>[4x]MGRENVLPVHNDVYEDFVFTTPYFQPESTFKSVPKLFSDILLGGVEWVYTTSESVLAYDYKLWYLWSGVSNLDESFDMFFNQYWALSLSTSVFQLFYAVILDRYLSVLFQNTPYTNDWFRMMLHSKETALIWLYHPELSWHINGLNQFFTYFYGGILEFVYFDKSNPDMCILVHTLWIHLLILFLIFTGFVTILFSFYGNPNTEENTIDSDYLAASGTVEAEKEITSIDDYLGLVFAIAYVFGVFFYVHGWTSMLSHAVLLLSCYSIIIMFLFILGMPTLLLYDFGIFFLAYLKGAGKYISSVAEMMFDYTACLVFYIRILAQWIRVVLMVVTFISLSHYVSDFDITNSALIGSENQSDSMNELNTNFSMTYYILTVLPGKFIYWIYEILHTFFVVCSQFVAFFAIVFWLFLFLYTFFIIEKHEDFFSKKREERKKKLKELWNLKN;>[12x]MIRNFHSLVKRVPRLALTPFFGFRTSMTLADKKLSTGEASVVLAEKIKGITQQNDITEYGTVISIGDGIARVFGLTKVQAGEMVEFKSGIRGMALNLETDNVGVVVLGNDRDIKEGDVVKRTGAIVDVPIGEAMCGRVFDALGNPIDGLGPLKTTQRARVEIKAPGIIPRQSVRQPMQTGIKCVDSLVPIGRGQRELIIGDRQTGKTAIAIDTILNQKEAFNTGDVKKQLYCIYVAVGQKRSTIANLVSILKQHDCMKFTIVVCATASDAAPLQFLAPYSGCAIGEFFRDNGKHALIIYDDLSKQAVAYRQMSLLLRRPPGREAYPGDVFYLHSRLLERAAKMNDSLGGGSLTALPVIETQAGDVSAYIPTNVISITDGQIFLETELFYKGIRPAINVGLSVSRVGSAAQIKAMKKIAGNLKLTLATYRELAAFSQFGSDLDAKTQQQLNTGERLVEMLKQNQYTPMKVEEQVCIIFAGVKGFLDALVTSEVLKFEKKFLEHVRTNHSALLKRIRDSGDLSEVDTNELNTIIPLFIQEGGFKLKAQ;>MHSTLRVFTKNNCLSFTNMNRFSTAAQVAQANYSKFRADYSASVAAFQQRIKTIEKENTGSMKKPMAKAYEHPYNSEHHPLNFSAVKIAETFHDFIGPEQVSPHYESFAMSRKFLLTFWGGFFVLNFGMATVDLNWIMKSTYIPWIFWFQLMYFYVEGKNSMFMPLLQRFYRRAAANEIFTMEAFYHENIENKLRNLMRITKGQLEYWDIHTSYGEIRADSINNFLANEYLRLQSHITSRALNILKQAQAYETMNQAALLQKLIDDATSAIDNALKGDKKAEVLARSLDSAIDGLSKGYMDYQNDPLLPLILSSIEANVKKITTLSAQEQANLIGLTAEQLKSIKENDVRARKEFLESQPKLDNNLKNIESVKKILATWGK[4x];>MITILDYLFLLDLNDDLTRKAVFEQVIIFIFIYCTMNFLAWSTVVELIWPTHFFNRRHSSSQEFIRFRTYTEVLLKISAYNDFFYVLNNYYYNQKLILKN[4x];>[4x]MSMLAKIAKNVVKTQALKNTTAAQTPSFQAPGNQDKILKWISTLSNKATTGESRSYCTQLSSLVSFYNKQHVEQIPTIDFNEWKSVISTQGLVDKVKENYESLIKEQYNTDAISKQISSASSKALDDIENELSFHAAIWLNAYADYTMFLFELEEYNDPNDYLMHENFDFFRGLETELEELTETHNYIPGAKDDVNLRGYLATQFAWGKKVISFYRHPADDFKCAKATKNMLGR;>[12x]MLSKALQRGIARAFSTTAKKEAPKTVKANGQVSQVIGAVVDVQFEGELPQILNALEVQGTQHRLVLEVAQHLGDSRVRTIAMDSTEGLVRGQPVVDTGLPISVPVGPGTLGRIMNVIGEPIDQRGPIKAAKLYPIHRDAPSFTDQATSAEILVTGIKVVDLLAPYARGGKIGLFGGAGVGKTVLIQELINNVAKHHGGYSVFAGVGERTREGNDLYHEMMDSKVISVKEGESRCALIFGQMNEPPGARARVGLTGLTVAEYFRDEEGKDVLLFVDNIFRFTQACSEVSALLGRIPSAVGYQPTLATDLGALQERITTTQKGSITSVQAIYVPADDLTDPAPATTFAHLDATTVLNRGLTELGIYPAVDPLDSTSRMLDPITIGEEHYTVARGVQKLLQDYKSLQDIIAILGVDDLSEEDKLVVARARKVQKFLSQPFFMSEVFSGIPGRFVNLKQNIASFKALLEGAGDEYPESCFYMKGDLEESLAAGRADALKSK;>[4x]MIHCLRNIRTVSALQSKISYNLGGGNKRKKTSGDLDNYDVLFVGANLGGICSNHFDKDTHGKYKCFVSFDQPINQIYSVRIPYEQQRVRKSEYIHFSKKSINQFTPSEMLAVKEILPEQNAVVLSSGRRIGYNQLVLATGLKHDFSQIKGFYEALEHPEHPVYANRDPETWRSAQHKYSKYISNFKSGDGYFCIPEYPYAGEVECFNFFVSDEVWKWAQHHGALSPKHTFTIVNANEKFVHYCDSADAFIKERLEKRGIRVEYNTKLLEVHQDGQKATFINTKTGEKSVRDYNNLYSIVPSKRQEFLDKAGLTNGNGLLNVDHQTLQHKKYKNIFGLGDAADLPTTKTFWAGWYQIAVVRNNVKRNLQGQTLNAHYDGFSKVPLFTGHQTLTYVAHSYGGVGNWQHLKHNNGGILAWMRYRSWAKGMAKKFQDFYNGARLGPPYHKVLKSFPELPGSPESQQSSGISKYFPTKTENKAAH;>MSLHEKMQTDYLWVKDHSQADSWAKARTHGYNYIAHTVPNKKERYEMIWRSMGKSTDWELEKFRLGKKFPDRGNKRRWFKNLFRLIKNPMGYIFWKTYKARLAKPSLIVTSMFIGFTLGFIKLKAQSIAYSKKQYATLRAGKNIEGSGQVHFGYHDQKWGMPAIPMFQLMYYELPGNSIVVNPCRNQNYRLYFEMRKKLGILPA[4x];>[4x]MINRSTAFISKNLRQANLTQSSLAMKTQYNQMGFSSDNPYNKRWEYKWKHSYYTYPRDYEHTEVRKPQDSKDVPPIYFAYYKDFVDRWLPGMNMWWQRRHRIFDKFNVYFLPGMSLFFYQFADLALGFKIMAAFPLFLAYTRIRDKTLDPDFKETYLRDMIYQNPEITKYFNEETIHVLDYEFEYLPGYLCPEKFPEYQNKTWQFFNTDTAQAEGFFKFGDVESGATMTLKFKTMPIPGKFRYQVGEPFYFYDLRAEIKCDGVYKEVVLVDEKESLKKIRPFLFLI;>[4x]MQVIRKHLAQKGLFNPFLFNRFSTQQDITSVPGDKPPAIEDSIHGKYAGVLFSSASSNKSLNKVAEDMKYFNQLYKESEVFKSFLNNVSLKRNQQRDIISALGKTNFNPATNNLLETLIENKRLDSLPKIAEKYMDYYRILNKQESITIISAQELTAAEKQKVEQGLKKGNANVQFTVVYQVDPAILGGLQMYSGNNFLDCSLLSRVNKLKTEIAKISF;>[4x]MQQRKKIYLRQKRKIYIQLKNKEKKKNNQFIQKREKMGYKIRNKSIFWTRAGWKNNWHPKNFNAPRPSYGEFTMGIRCRNDHHSFLRYVQTYRNMSRHCKQY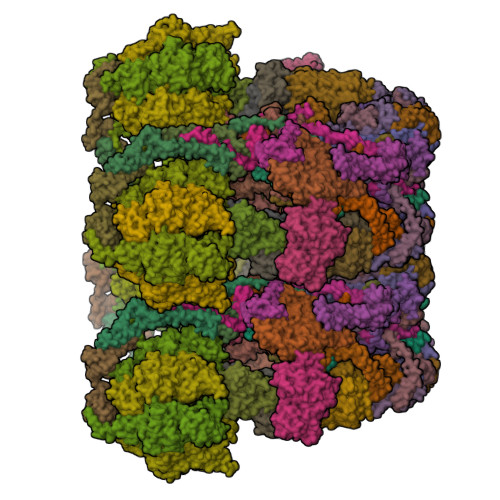FLGDKQLEETFILGLRSLFLVPYDSQCLTDQIKHGGERRFVDQLDRDFELISYNTHPYQLFTYTVRNEHLAWKNEQYEKIQKGEKTFEQELLDYLDEQVLAEKAKLRDGQNFSIERMTEIALHVFRKARAGKVRPAQDVRGPDGNVNDFLEQRRPFEHPNPTGVTH;>[40x]MLLVKAVKVLVMGGCMLPIAFGALGTGVLFAGFNVALSRNPEETESLFNNTLMGFALIETFIFMSIGLGFFVLFAA;>MNPIQKAWLKILEPVSYVINEKMAKRTGIIGKLGRFFAIGPREYGVHPINRMFIFMNRKYMAFQAVALHRYSFVKSLTHNGFHMLRVFRHFAFVLPATVLAGLGLFVYWGDDNKCYSPDRFPYLKKRAGDMALPLNSLNQRTSAHYIEINAIYGAEMMKRYHKVWENIIEERSKATDQEKKTRYAHPSYQYSPLPVVSIPNVLNPLNLQ[4x];>MSENKAPGQIYAYDIHNTHYPYVNIKQDSQTQLLASFRRSIASINPFSYRQVPSQDRAAFGLRWGNAWYAPNPYPNGIHFDRVFPTHYDPLAETNRTKANLQLIKYAPGNYSTLVVTSEKLPRPCIRTIQNYRRCQMVNGTEKCNSEAQDILAICPNWALDHMKEKVRFYTKALAINNQTYIRAMQVEEYNQGRTVADVAPKTWIHGTRQHLRPDTMWADDRYTNITQTEINEAIKRVEARKAREHEKKPVEQANVNANTGEQPVRVEKSLYP[4x];>MWYKYFSKQSWNLRVWRKANLKYNQDDFGMTQPKYIARFGDFRFRLVRTEGALRGCMFFVGFGCFSIINYLYGRYGYIINESSQKRAAQDLLDNDMAADKILFKNRVGAPTRPLRSLDDMMAFLSGSATYDQLADYASYNHAMDVNQDQQAGLDSWMSEKDKNMVKYYQRSLGKKVEGI[4x];>[4x]MPVKEGQAKLWFSTKEEADAYDDKMISNIELKSQDYEDENFSPVFNRKTQEYFLEPSEKFKSDFAELLRPLRSLSFNQVVDRYVLIPPNHTFYRNWTYEKFLGGFGLSYLILRELPLRNFYARVFVMYAFAAKVLDHLGNPFPFSGHGQIVAAADRWNHWDVRCYDNVMKALKYIRIPTVQNNIPEATRWYGRQPGHLLRADTYWIPNLVSQRFAKHQPAHWDGTQNMPIFRLADPKHKDSYMVQFR;>MDNYFTAITLLGLRDQNLPPFKDARLQRYKSIKKMIDLIETTTKLAPPMPVELFMLNPTDPEWDDDMTYPTITHATALYKSSALAGNLFLYAYNYNNFTANIRLRTMRYLFPVVSLAIFGNIYWDYRSQLVKVNLFDEYIQARAQELVKQNEYLLEHEDVKRYVWWYEDLKETLARVHRQANNHKACDFKDSEIILQDFIRRYTNPKDNLPIKFHPQGQTF[4x];>MEGFIQNKRKKEKEGEEEEESKEKRKQINQLNKQKQEEEKIYQQKKDQKRKKYLYQRKEMTIFAETWEASEYQYRNKANLKTLPVNHLGKLAELKFDFVEYKAHQLIACHLYERMTIHCMNQYGLFKDFYRPECLDAQYYFKTCVELNAAYGIQKKFFPEHFVGSPYARPVPQFQQLGL[4x];>[4x]MKQKINKLLKNKGVQDKYKYLSKLILLDQEIKGKIKRKNKKEKQKRKNKLILEEMQNTTNIVHVPVHMGHTHYFDYIDSFPKLKEGPTLEENHITNQKILREQLISGQQGLEQNLCLRNCFKLSQKRYIEFCLDRKCGGADFQRAATILGYTKN;>MSNIFLELQDGDKTVYTHTSLIEESKQEQIQAIYDKVPQWTNGGRFLGFWLSMEAVNRVQSVAKLPIYYRAGIVATSTLLGGLVSSLVFWKSGNENQVAKLANGAPVYLKKWEVPELSKLYFFLDDDNNFKPSLNHHAVTQGRQYYKIYQHN[4x];>MFRNILSLVTKPSKLSQKTFYNFAAAKNEVQVSKKQQQAGAKRDLTQYVEGQIVNRNQLTLKKQEDIEQYVLKLVRGYFRTTNKQGLNINSVLQDHGLDEFDSIELAMQVEEDLGYVISAETIPVLNKVKHFVNYINHVEQFKAENGKAPIA[4x];>MSQDPKIVNPQLWPNPNKLRFADLYKYQGVEMKKINDSIKNYKAAKFYIGGILGGCLVFKFFIDAAVDKYIFGENGNGGKFLEMQTINSNYDYYYNRQFQRMRYLTEDPAGDDPLQKTKDEHLVDLGFIPKVFGANVEVRKRAPHDKYL[4x];>[4x]MNSLSSKKANSLVFKSIRNFTLQWGSLAERPMVDRVMSTSTWPVPYYQRLFKAYPIREKKDKMSLLLSDIDIDDTNWYQAKDFLRGSFRGRQIVDYVENNIASNTYILIQQDVANMAKAYVHDICGYIDVANKENVRILSKGDLI;>MFTRFVTQPTLLTQTQRALFSALTKKQKMEVTLRTPYKEYLANFDGFSRITAKTNEASLVIQNKTPASLYVLPPGPLKIRFTSEVKNVSGDFLHTGGWVIVHADNTCEINVMDLFDRKEVRADQFEKGNIQDLDTLAGKYAAKSRKSTVRLFTKATTQ[4x];>MCIEFAFKKAGIPIVRNFLHSTEGVIYGLPQRVQRNLAINYTVKQYKEGKAVSAKTIKTLQEAFPSKGDTK[4x];>[4x]MFGLASKGFINTSLVMVPQMNFGANLKQLKIRMKAIGSIKKITKAMKMVAASKMKAETSRLENGRNFAVGSVQKMLENESYVQKKKSTTAPKSTLLVPITSDKGLCGSVNSSIVREVKRLALNNRSAFGLLPVGEKGSSGLSRPFPDLLKSSIVNIQNVNFPTAAAIAHQVSTQGAGYDQVTLIYNHFKNAISYVVKHQELLPRAQFLNLFKYVTRHEAVEPELEYSKNYFFELYMASSVYNALLNSSASEQASRMNAMENASKNAGEILSKLTLDYNKARQAKITMELIEIISGASIV;>MNRSVNIAKNLIQTYRAMSVQSRFAFSTREEEWLDKRTKSQEKVYFDQEDRKAMKRLLEKLNTTSKFVEDSEYLAPQNLEVENILKRYHINYTQALIDELVDWKTGKN[4x];>MKMEYLQSEEKKDAINKQIHKKEEKEEKEIKIKRKNKVKQRIQIINQIKKYIEAKQQKKQIQSKNQRKYKGRMINTRKQVFKCLWGAQPAYNFSRIINHLRGDPVYQDNTKDVSLRGTFLRGKYDDLPTMIFFTEACDLTANWIPFFTNPQYDILAHRNVWLLNPRNFGNSDRHPSFDLQEMSDDVMRFMYSQKISMATLGGHGIGGKIALAVGCYHAERVTGVFSIDSSPMDQRYHEAFKEFKGYVNALTEINFKTWSDKDVKVFLKENIKDPKWRSIFTNNISKNAKTQSDSFNFEINYLNHNLNFNKADSLGNWAVKNGIYTGRAHFIFPEYSRWVHLATNTLPMHKVCARVKGFGHDIFYVQGDENPLNHWVYDFENYANVVASKLNKFLHSYDGVHALLKDRTEIGNFMIPDRIKSRNDSKHIYGDYSPAHLHHNWRFNHIYEKHDELDKKLNEQ[2x]> SNAMTNRYTTLFANLEKRNEGAFIPFVTIGDPNKALSFEIIDTLVSSGADALELGIPFSDPLADGPTIQEANIRALESGITPKDCFDILTKIRAKYPHIPIGLLLYANLVYANGIENFYQKCLDAGVDSILIADVPAHESKEFRDIAKKVGIAQIFIAPPDASESTLKQISELGSGYTYLLSRVGVTGTETAANMPVEDVLTKLREYNAPKPVLGFGISKPEQVQQAIKAGAAGAISGSATVKIIQNNISNKQKMLNELTYFVKEMKAATLN;> MSKLNAYFGEYGGQFVPQILVPALDQLEQEFIKAQADESFKQEFKELLQEYAGRPTALTKTRNIVKNTRTKLYLKREDLLHGGAHKTNQVLGQALLAKRMGKKEIIAETGAGQHGVATALACALLDLKCRVYMGAKDVERQSPNVFRMKLMGAEVIPVHSGSATLKDACNEALRDWSANYSKAHYLLGTAAGPHPFPTIVREFQRMIGEETKQQMLAKEGRLPDAVIACVGGGSNAIGMFADFIDEKNVKLIGVEPAGKGIETGEHGAPLKHGKTGIFFGMKAPLMQNSDGQIEESYSISAGLDFPSVGPQHAHLLAIGRAKYASATDDEALDAFKLLCKKEGIIPALESSHALAHALKLAYEDPNKEQLLVVNLSGRGDK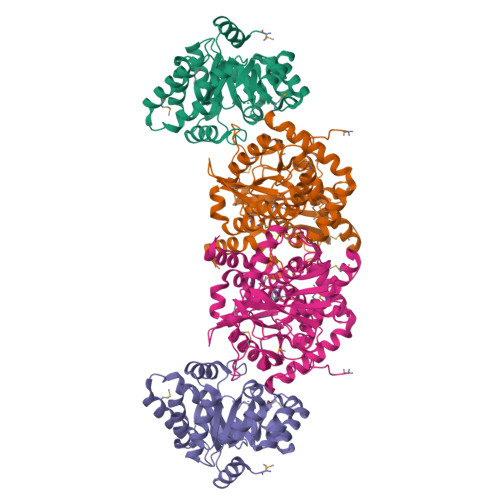DIFTVHDILKEKGEI>ATKVAVAGASGYAGGEILRLLLGHPAYADGRLRIGALTAATSAGSTLGEHHPHLTPLAHRVVEPTEAAVLGGHDAVFLALPHGHSAVLAQQLSPETLIIDCGADFRLTDAAVWERFYGSSHAGSWPYGLPELPGARDQLRGTRRIAVPGCYPTAALLALFPALAADLIEPAVTVVAVSGTSGAGRAATTDLLGAEVIGSARAYNIAGVHRHTPEIAQGLRAVTDRDVSVSFTPVLIPASRGILATCTARTRSPLSQLRAAYEKAYHAEPFIYLMPEGQLPRTGAVIGSNAAHIAVAVDEDAQTFVAIAAIDNLVKGTAGAAVQSMNLALGWPETDGLSVVGVAP[8x]

The L-arginine biosynthesis pathway consists of eight enzymes that catalyse the conversion of L-glutamate to L-arginine, appears to be attractive target for anti-Tuberculosis (TB) drug discovery. The arginine biosynthesis pathway consists of eight different enzymes ([Fig fig1]) all considered to be essential for *M. tuberculosis* growth *in vitro*. In this work, the ligandability of four enzymes of the pathway ArgB, ArgC, ArgD and ArgF is explored using a fragment-based approach. In conclusion, using a fragment-based approach, we have discovered inhibitors that bind to novel sites in ArgB and ArgF and to the active sites of ArgC and ArgD, which in case of ArgB show on target activity against *M. tuberculosis*.

Additionally, structures were solved with 4 fragment binders, occupying either of the two distinct pockets: the substrate-binding ([Fig fig2] and [Fig fig2]) and the NADP(H)-binding pockets ([Fig fig2] and [Fig fig2]). Enzymatic assays revealed that 2 mM NMR322 inhibited ArgC activity by 45% whereas 2 mM NMR571 caused a 37% inhibition. Although the thermal shifts obtained for NADP(H)-binding pocket fragments NMR401 and NMR863 were higher than those for substrate-binding pocket fragments NMR322 and NMR571, the SPR binding response for the latter was better and positively correlated with percentage inhibition of enzymatic activity (**[Table tbl2]**). Our results further show that in the case of ArgC there are two possible strategies to develop inhibitors, with one targeting the cofactor binding site and the other the substrate binding site. It is not clear at this point which strategy has the highest potential to result in potent inhibitors.>MTNRLVLSGTVCRAPLRKVSPSGIPHCQFVLEHRSVQEEAGFHRQAWCQMPVIVSGHENQAITHSITVGSRITVQGFISCHKAKNGLSKMVLHAEQIELIDSGD[2x];> MPVAHVALPVPLPRTFDYLLPEGMTVKAGCRVRVPFGKQQERIGIVVSVSDASELPLNELKAVVEVLDSEPVFTHSVWRLLLWAADYYHHPIGDVLFHALPILLRQGRPAANAPMWYWFATEQGQAVDLNSLKRSPKQQQALAALRQGKIWRDQVATLEFNDAALQALRKKGLCDLASETPEFSDWRTNYAVSGERLRLNTEQATAVGAIHSAADTFSAWLLAGVTGSGKTEVYLSVLENVLAQGKQALVMVPEIGLTPQTIARFRERFNAPVEVLHSGLNDSERLSAWLKAKNGEAAIVIGTRSALFTPFKNLGVIVIDEEHDSSYKQQEGWRYHARDLAVYRAHSEQIPIILGSATPALETLCNVQQKKYRLLRLTRRAGNARPAIQHVLDLKGQKVQAGLAPALITRMRQHLQADNQVILFLNRRGFAPALLCHDCGWIAECPRCDHYYTLHQAQHHLRCHHCDSQRPVPRQCPSCGSTHLVPVGLGTEQLEQTLAPLFPGVPISRIDRDTTSRKGALEQQLAEVHRGGARILIGTQMLAKGHHFPDVTLVALLDVDGALFSADFRSAERFAQLYTQVAGRAGRAGKQGEVVLQTHHPEHPLLQTLLYKGYDAFAEQALAERRMMQLPPWTSHVIVRAEDHNNQHAPLFLQQLRNLILSSPLADEKLWVLGPVPALAPKRGGRWRWQILLQHPSRVRLQHIINGTLALINTIPDSRKVKWVLDVDPIEG

PriA, which is the only replication restart factor found in all bacteria, acts as a “first responder” protein, recognizing abandoned DNA replication forks in a structure-specific manner and recruiting other factors needed for replication re-initiation. PriA is a 3′−5′ DNA helicase that comprises six domains: a 3′ binding domain (3′BD), a winged-helix domain (WH), two helicase domains (HD1 and HD2), a cysteine-rich region (CRR), and a C-terminal domain (CTD). PriB, which is a homodimeric paralog of ssDNA-binding protein (SSB), stimulates the DNA unwinding activity of PriA and forms a stable complex with PriA bound to replication forks that have ssDNA lagging strands. Binding of PriA to a replication fork triggers PriB docking, with PriB binding ~100-fold tighter to the PriA/replication fork complex than to PriA alone.

To investigate the molecular mechanisms underlying DNA replication restart initiation, we determined a 3.2 Å global resolution structure of the E. coli PriA/PriB/replication fork complex using cryogenic-electron microscopy (cryo-EM) single-particle analysis. The DNA replication fork included a 25-base pair parental arm, a 15-base pair leading strand, and a 15-nucleotide ssDNA lagging strand (Fork 5). Analysis of this class resulted in a 3.2 Å global resolution map that included EM density for a PriA monomer, a PriB dimer, and each arm of the replication fork DNA substrate. In addition to lagging strand binding, PriA binds the leading strand and parental arms of the replication fork to create a multi-point binding surface that recognizes structural features characteristic of abandoned replication forks and D-loops. Replication fork binding induces a dramatic conformational change in PriA in which the CRR domain pivots ~85° and the HD2 domain rotates ~15° to create a pore enclosing lagging strand ssDNA. Well-resolved EM density showed lagging strand ssDNA from the replication fork threaded through the pore, with 8-9 nucleotides stretching from the replication fork junction to the end of the pore. In addition to opening a ssDNA-binding pore, a second notable impact of PriA-CRR pivoting is that it exposes a surface of the domain onto which PriB docks, directly linking PriA replication fork recognition with PriA/PriB protein complex formation. PriA/PriB interaction in this arrangement buries ~1600 Å2 of surface area (calculated using the PISA server) and is supported by a network of well conserved and electrostatically compatible residues from both proteins. These include Asp438, Ser481, Thr482, and His483 from PriA interacting with His26, Glu39, Arg44, and His81 from PriB. Binding to the CRR places PriB at the edge of the PriA pore entrance where PriB directly engages ssDNA extending from PriA.> MGKALVIVESPAKAKTINKYLGSDYVVKSSVGHIRDLPTSGSAAKKSADSTSTKTAKKPKKDERGALVNRMGVDPWHNWEAHYEVLPGKEKV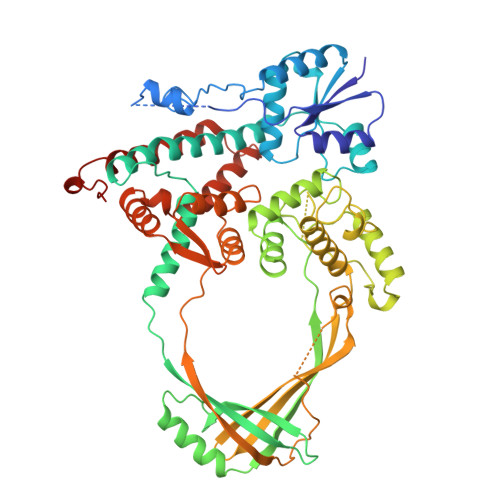VSELKQLAEKADHIYLATDLDREGEAIAWHLREVIGGDDARYSRVVFNEITKNAIRQAFNKPGELNIDRVNAQQARRFMDRVVGYMVSPLLWKKIARGLSAGRVQSVAVRLVVEREREIKAFVPEEFWEVDASTTTPSGEALALQVTHQNDKPFRPVNKEQTQAAVSLLEKARYSVLEREDKPTTSKPGAPFITSTLQQAASTRLGFGVKKTMMMAQRLYEAGYITYMRTDSTNLSQDAVNMVRGYISDNFGKKYLPESPNQYASKGNSQEAHEAIRPSDVNVMAESLKDMEADAQKLYQLIWRQFVACQMTPAKYDSTTLTVGAGDFRLKARGRILRFDGWTKVMPALRKGDEDRILPAVNKGDALTLVELTPAQHFTKPPARFSEASLVKELEKRGIGRPSTYASIISTIQDRGYVRVENRRFYAEKMGEIVTDRLEENFRELMNYDFTAQMENSLDQVANHEAEWKAVLDHFFSDFTQQLDKAEKDPEEGGMRPNQMVLTSI4-({2-[(4-chloro-3-{[(2S)-1-methylpyrrolidin-2-yl]methoxy}phenyl)amino]-1,3-benzoxazol-5-yl}oxy)-N-methylpyridine-2-carboxamide 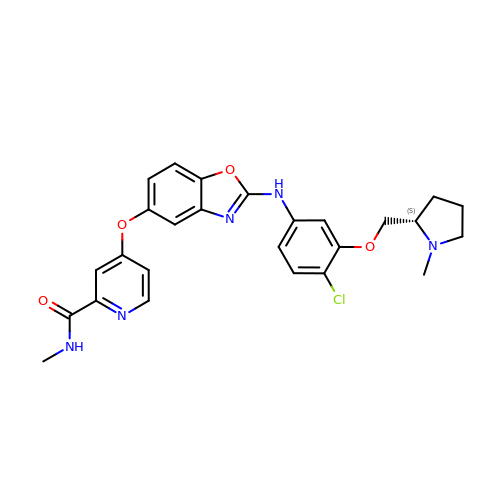| C26 H26 Cl N5 O4 | KMNCFOUKJYOZIF-KRWDZBQOSA-N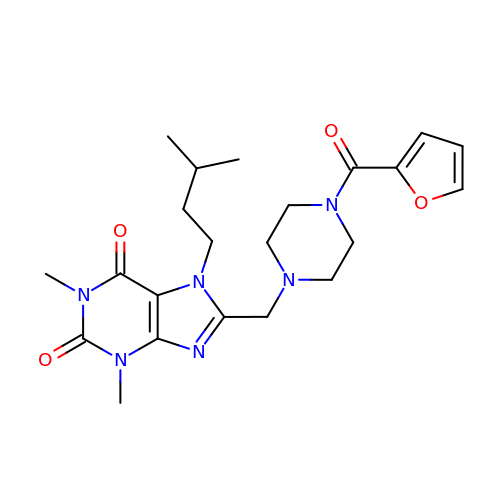8-{[4-(furan-2-ylcarbonyl)piperazin-1-yl]methyl}-1,3-dimethyl-7-(3-methylbutyl)-3,7-dihydro-1H-purine-2,6-dione | C22 H30 N6 O4 | AGUUKKXWABRVBZ-UHFFFAOYSA-N> TELPLATPCDEEACKLPDCRCSSTNIPGGLRARDTPQFVTVTFDDGINVINIETYREVLYGRSNSNRCPAGATFYVSHEYTNYQLVNELYNRGFEIALHSISHRTPQAFWADATYQNLVQEIGDQKRQMAHFASIPASAIKGVRIPFLQMSGNTSFQVMADFDLLYDCTWPTTALTNPGLWPYTLHHESIQDCIIPPCPTASIPGPWVLPMISWRDLNNFPCSMVDGCFFTPDRTDEEGWFKFILTNFERHYLGNRAPFGFFVHEWFISSNPAI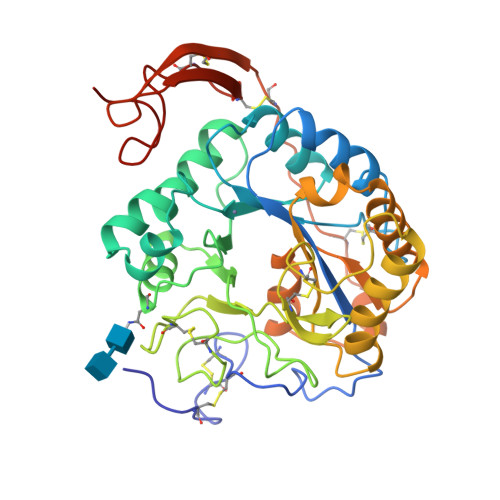KRAFVRFMDIINNLNDVFMVNSAEVIDWVKNPVPIDRYRQQQCKFTMPSICRPSFCGPLTGTHNQLSYYMTICNTCPRNYPWVGNPLGQHHHHHH>EDPSLDRPFISEGTTLKDLIYDMTTSGSGSGLPLLVQRTIARTIVLQESIGKGRFGEVWRGKWRGEEVAVKIFSSREERSWFREAEIYQTVMLRHENILGFIAADNKDNGTWTQLWLVSDYHEHGSLFDYLNRYTVTVEGMIKLALSTASGLAHLHMEIVGTQGKPAIAHRDLKSKNILVKKNGTCCIADLGLAVRHDSATDTIDIAPNHRVGTKRYMAPEVLDDSINMKHFESFKRADIYAMGLVFWEIARRCSIGGIHEDYQLPYYDLVPSDPSVEEMRKVVCEQKLRPNIPNRWQSCEALRVMAKIMRECWYANGAARLTALRIKKTLSQLSQQE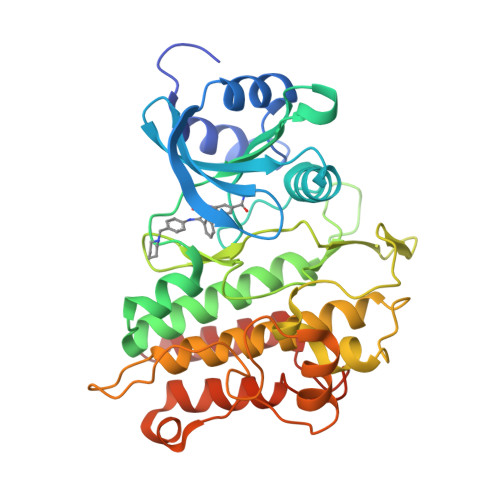GIKM[5x]>[2x]MTKPYVRLDKNDAAVLLVDHQAGLLSLVRDIEPDKFKNNVLALGDLAKYFNLPTILTTSAETGPNGPLVPELKAQFPD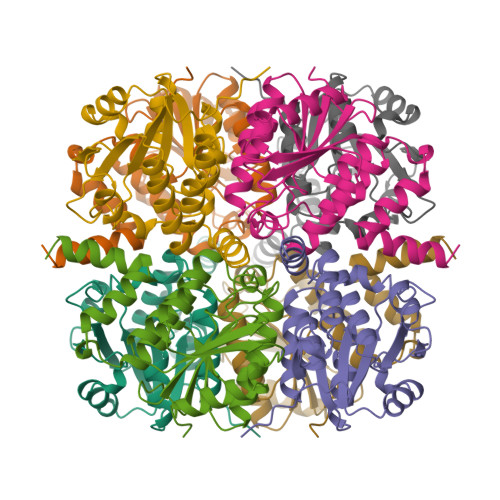APYIARPGNINAWDNEDFVKAVKATGKKQLIIAGVVTEVCVAFPALSAIEEGFDVFVVTDASGTFNEITRHSAWDRMSQAGAQLMTWFGVACELHRDWRNDIAGLATLFSNHIPDYRNLMTSYDTLTKQK> EFLPNQRRSNVTSHVETYYSVDGATHAEKSKALKADGYRIVSLSSYGSPDSANYAAIWVQEEGPSFEIIHDADEATYNSWLQTWKSRGYVSTQVSATGPAENAVFAGVMENINVANWFQSCELENPWAFSNTTGNVDVVVKGFRMFGTPEERRYCILGHENVGNEQTTIQYSTPSFTVNFASTFEAETTKRFWRPSRLFLSEDHIITPSFADTSVGKWSHAVDLTKAELKEKIETERAKGLYPIDIQGGGSGSSERFTV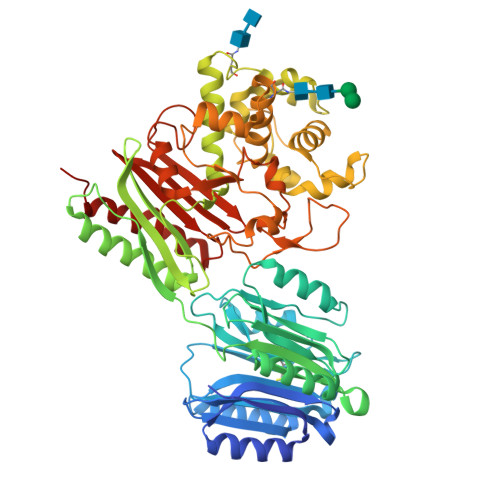VFAERTSPKPRQWNVRGEITGFEDNKAAEEEVDSIMRRFMEKNGVRQAQFAVALEGKTIAERSYTWAEDDRAIVEPDDIFLLASVSKMFLHASIDWLVSHDMLNFSTPVYDLLGYKPADSRANDINVQHLLDHSAGYDRSMSGDPSFMFREIAQSLPTKGAKAATLRDVIEYVVAKPLDFTPGDYSAYSNYCPMLLSYVVTNITGVPYLDFLEKNILDGLNVRLYETAASKHTEDRIVQESKNTGQDPVHPQSAKLVPGPHGGDGAVKEECAGTFAMAASASSLAKFIGSHAVWGTGGRVSSNRDGSLSGARAYVESRGTIDWALTLNTREYISETEFDELRWYSLPDFLSAFPIAG Among them are the ubiquitous surface proteins (Usps): A1, A2, and A2H, which all belong to the trimeric autotransporter adhesin family. They bind extracellular matrix molecules and inhibit the classical and alternative pathways of the complement cascade by recruiting complement regulators C3d and C4b binding protein. TAAs are anchored in the bacterial outer membrane by a 12-stranded β-barrel (the translocation domain) comprised of four strands from each monomer, from where the passenger domain is exposed to the extracellular environment. The passenger domain consists of an N-terminal β-strand head domain followed by the neck domain and a coiled-coil stalk.

In this study, we present the crystallographic structure of UspA1299–452, which contains the putative C3d binding site. The asymmetric unit of the crystal contained one trimer of UspA1299–452, as is typical of a trimeric autotransporter adhesin. It consists of part of the neck domain (residues 299–336) and the stalk (residues 337–452). The neck domain of UspA1299–452 is a long neck containing, towards its end, the characteristic DAVN motif that mediates the transition from the left-handed parallel β-roll headgroup to the α-helical stalk. The stalk domain is a left-handed coiled-coil built mostly from heptad repeats with the typical arrangement of repeating hydrophobic (h) amino acids separated by polar (p) residues in the seven-residue abcdefg pattern hpphppp. There are, however, two disruptions from the heptad pattern: after Gly396 and Gly442 in the d position, there is a Leu that occurs structurally at position a, instead of the canonical polar amino acid at position e to complete the abcdefg heptad pattern. In addition to Leu, there are another three amino acids (LeuAspLeu) inserted in these sites making them an 11-residue pattern. This changes the periodicity of the coiled-coil from heptad (7-residue pattern) to hendecad (11-residue pattern), which is consistent with the daTAA server predictions. The side chains of Asn347, 375, 382 and 414 in the d positions face the central core of the trimer and the amide nitrogens of their side chains coordinate chloride ions, forming characteristic N@d layers; the distances of those interactions range from 2.90 to 3.61 Å, as expected. Cl− coordinated by amide nitrogens of Asn414, in contrast to Cl− coordinated by other Asn, have only 50% occupancy, as there was strong negative (Fo-Fc) density after refinement with 100% occupancy (more details in Discussion). We performed multiple binding studies between recombinant C3d and UspA1299452, but were not able to demonstrate saturation binding; the Kd appears to be 140.5 ± 8.4 μM, which is not consistent with physiological concentrations of C3.

>[3x]KTGNGTVSVGKKGKERQIVHVGAGEISDTSTDAVNGSQLHALATVVAQNKADIKDLDDEVGLLGEEINSLEGEIFNNQDAIAKNQADIKTLESNVEEGLLDLSGRLLDQKADIDNNINNIYELAQQQDQHSSDIKTLKNNVEEGLLDLSGRLIDLVPR> SSIFLLSNVSEDAAQLAEELVREISKKEGTEVRFEKDDGFLT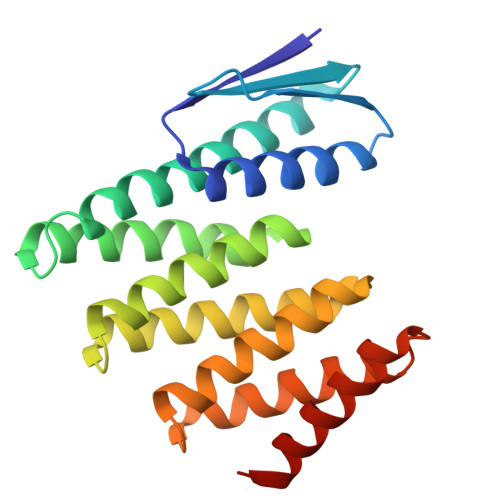IEVKNLSEERLREIAKALQLIVDVANAERVVRERPGSNLAKKALEIILRAAEELAKLDLKASLKAAVRAAEKVVREQPGSNLAKKALEIILRAAEELAKLPDPEALKEAVKAAEKVVREQPGSELAKKALEIIERAAEELKKSPDPEAQKEAKKAEQKVREERPGS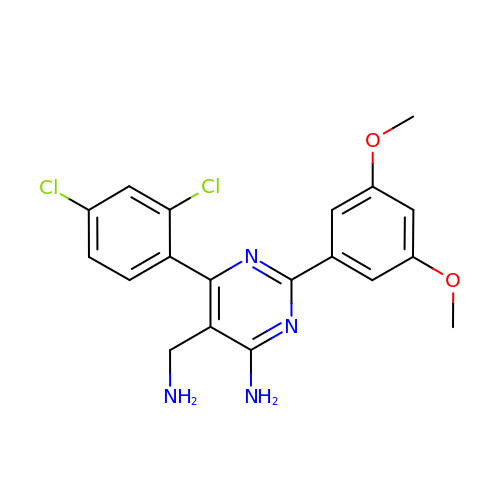5-(AMINOMETHYL)-6-(2,4-DICHLOROPHENYL)-2-(3,5-DIMETHOXYPHENYL)PYRIMIDIN-4-AMINE | C19 H18 Cl2 N4 O2 | RCJFINNFYUNFGH-UHFFFAOYSA-N(2S)-3-{4-[3-(4-{[(2R)-2-hydroxy-3,3-dimethylbutyl]oxy}phenyl)pentan-3-yl]phenoxy}propane-1,2-diol | C26 H38 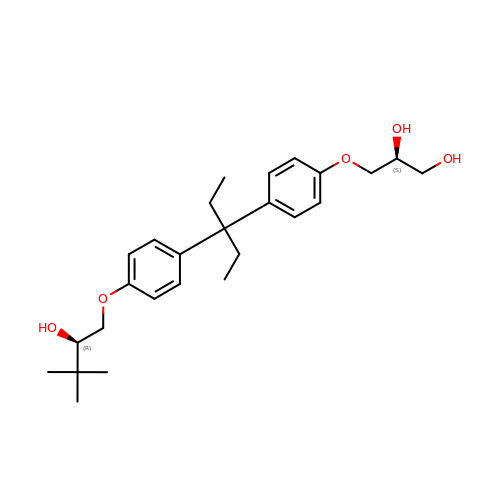O5 | HPEKDMRENBLBLH-URXFXBBRSA-N>MSKNRSSLQSGPLNSELLEEQKQEIYEAFSLFDMNNDGFLDYHELKVAMKALGFELPKREILDLIDEYDSEGRHLMKYDDFYIVMGEKILKRDPLDEIKRAFQLFDDDHTGKISIKNLRRVAKELGETLTDEELRAMIEEFDLDGDGEINENEFIAICTDS[4x];>[2x]GPLGSKLNDILHVYEKSKERELQSQLFNAWRNRFCFYTEECNIQAISKRNYQLEKMVLKKFRERL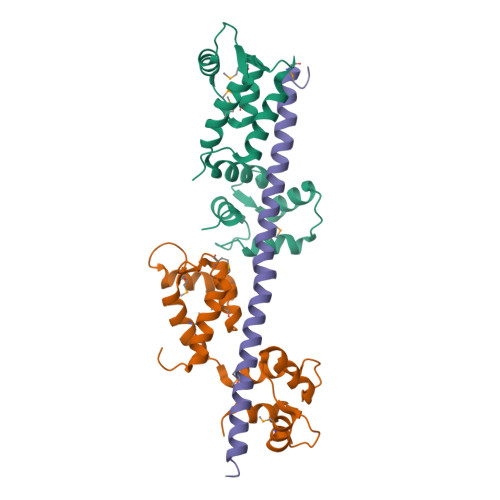LEIVKSEE> MASQPAQKSAYGKMLEELLGPKQTYESVTRTIGDIVLTPIRKTPWGWPVGFVIAALGLLMYLFSLAVLFTVGVGVWGINIPVAWGFDIINFVWWIGIGHAGTLISAILLLFRQDWRTSINRAAEAMTIFAVACAGIYPLVHTGRPWLDYWMLPYPGTLGMWPQFRSALEWDVFAISTYATVSILFWYLGLIPDLASLRDRATNIWVKRFYGFLALGWRGGARDWNRYEVASLILAGLSTPLVLSVHSIISLDFAISQLPGWHVTVFPPYFVAGAVYCGFAMVILLLVPLRRWYKLHDLITIKHFDLMGKVMLASGLVVAYGYFAEIFYAWYSANIYEYFLITNRTMGPYAWSYWALIVLNVAIPQLLWFKRFRVSLPWLFFISICINIGMWFERWVIIVLSLHRDFLPSSWGYYTPSVWDISLYAGSFGWFFFLFFL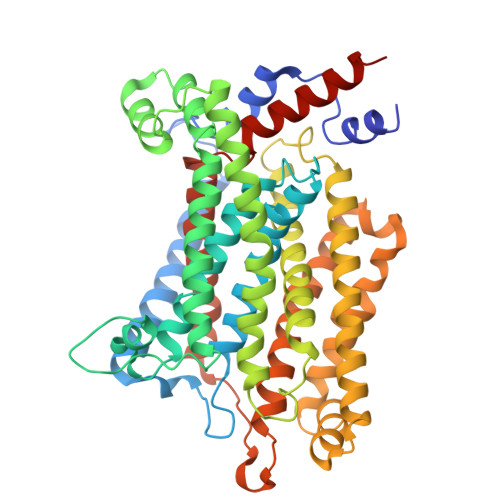FIRLLPAISIFEVRDLVHKTETEKALAHGSAGHH>SVEEIRLPRAGGPLGLSIV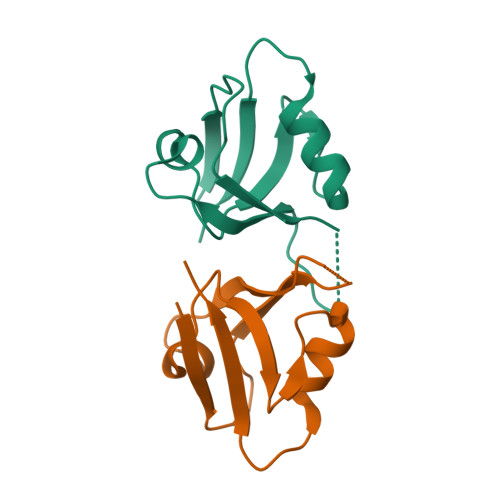GGSDHSSHPFGVQEPGVFISKVLPRGLAARSGLRVGDRILAVNGQDVRDATHQEAVSALLRPCLELSLLVRRD[2x]One group of metal ion efflux transporters that regulates metal ion homeostasis and can be found in all domains of life is the Cation Diffusion Facilitator (CDF) protein family. One of the most highly conserved and abundant integral MM proteins is the CDF transporter MamM. MamM was recently proposed to function as a magnetosome-directed iron transporter required for iron biomineralization since its deletion abolished magnetite biomineralization and mutation of residues within the conserved TMD metal-binding site resulted in alterations of magnetite crystal size, morphology and even mineral phase. To summarize our results we present an alternative model for the CDF CTD mode of action, in which we propose that upon metal cation binding, the CTD induces conformational changes towards a tighter and more compact fold which allows the activation of iron transport through the TMD.

To test this hypothesis, we combined the D249A point mutation at the central binding site and the H264A mutation at peripheral sites. Although no cation binding was detected for the resulting double mutant, D249A + H264A, by ITC in vitro it still produced magnetite particles in vivo. However, magnetite formation was severely affected in the D249A+H264A mutant as a significant non-additive decrease of the magnetic response, the average particle numbers and the average crystal sizes were observed. In addition the D249A+H264A double mutant showed a drastically delayed formation of magnetite during iron induction experiments. These results suggest that proper sensory and regulatory activity of the CTD can be achieved through a single type of binding site, either the central or the two peripheral sites, to allow proper activation and transport of MamM TMD. Therefore, the reduced magnetite formation reflects decreased MamM activities caused by less (e.g. MamM D249A) and/or shorter (e.g. MamM D249A+H264A) TMD activation events. To confirm that these observed phenotypic differences are due to true transport function alternations, we also examined the expression levels of all MamM mutants, their ability to stabilize MamB expression, performed MD simulations for dimer stability evaluation and determined their CTD structures. (ii) All mutants exhibited an apo-MamM CTD-like behavior along the MD simulations (see Fig. B in file S1 for representative MD simulations), and (iii) an absence of structural differences was observed.

> GSHMEAVQNRIVEAAERVPGVRGVIHLRARYVGQDIWAAMIIGVDPENTVEQAAEICEAVQAAVCGKIRRIESLHVSAEAREIGDTTKPSFSDQPLSFDEVMLSKVDN>[4x]QQCGQTAPLINERLSYMKDVAGYKAENHLPIEDRIQEEKVINS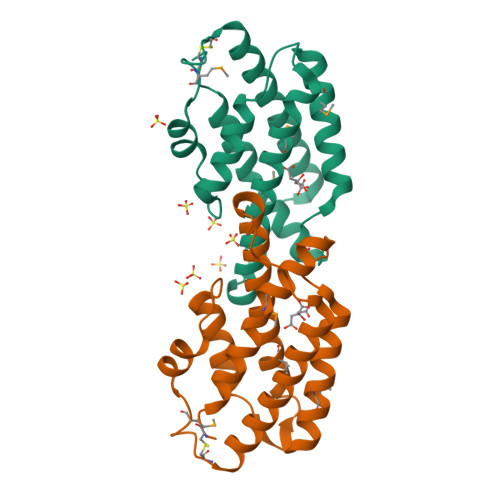AMAQAESLGLNGESIKPLMVAQINAAKAIQYRYRADWLSQPEPGWQPKPLDDVRANIGELSTKILEQIAEELKTCKPAEMGDKAHFINTIRQHNLTSADVEAIFSTFNQVKLK> VDCSEYPKPACTTEYRPLCGSDNKTYGNKCNFCN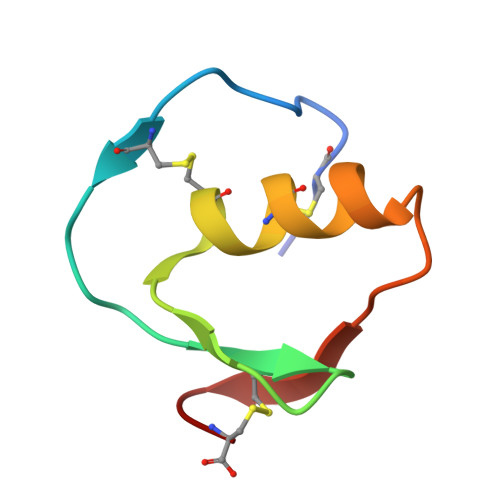AVVESNGTLTLSHFGKC> IVGGKVCPKGECPWQVLLLVNGAQLCGGTLINTIWVVSAAHCFDKIKNWRNLIAVLGEHDLSEHDGDEQSRRVAQVIIPSTYVPGTTNHDIALLRLHQPVVLTDHVVPLCLPERTFSERTLAFVRFSLVSGWGQLLDRGATALELMVLNVPRLMTQDCEASSPGKITEYMFCAGYSDGSKDSCKGDSGGPHATHYRGTWYLTGIVSWGQGCATVGHFGVYTRVSQYIEWLQKLMRSEPRPGVLLRAPFP;> ANAFLEELRPGSLERECKEEQCSFEEAREIFKDAERTKLFWISYSDGDQCASSPCQNGGSCKDQL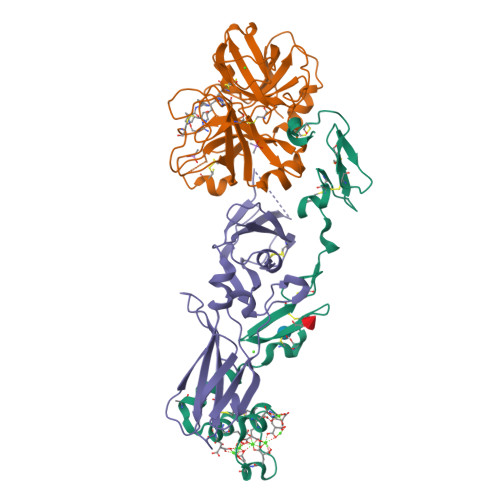QSYICFCLPAFEGRNCETHKDDQLICVNENGGCEQYCSDHTGTKRSCRCHEGYSLLADGVSCTPTVEYPCGKIPILEKRNASKPQGR;> SGTTNTVAAYNLTWKSTNFKTILEWEPKPVNQVYTVQISTKSGDWKSKCFYTTDTECDLTDEIVKDVKQTYLARVFSYPAGNVESTGSAGEPLYENSPEFTPYLETNLGQPTIQSFEQVGTKVNVTVEDERTLVRRNNTFLSLRDVFGKDLIYTLYYWKSSSSGKKTAKTNTNEFLIDVDKGENYCFSVQAVIPSRTVNRKSTDSPVECMGQEKGEFRE> EKEEAIFRSAEMALVQFYIPQEISRDSAYTLGQLGLVQFRDLNSKVRAFQRTFVNEIRRLDNVERQYRYFYSLLKKHDIKLYEGDTDKYLDGSGELYVPPSGSVIDDYVRNASYLEERLIQMEDATDQIEVQKNDLEQYRFILQSGDEFFLKGDNTDSTSYMDEDMIDANGENIAAAIGASVNYVTGVIARDKVATLEQILWRVLRGNLFFKTVEIEQPVYDVKTREYKHKNAFIVFSHGDLIIKRIRKIAESLDANLYDVDSSNEGRSQQLAKVNKNLSDLYTVLKTTSTTLESELYAIAKELDSWFQDVTREKAIFEILNKSNYDTNRKILIAEGWIPRDELATLQARL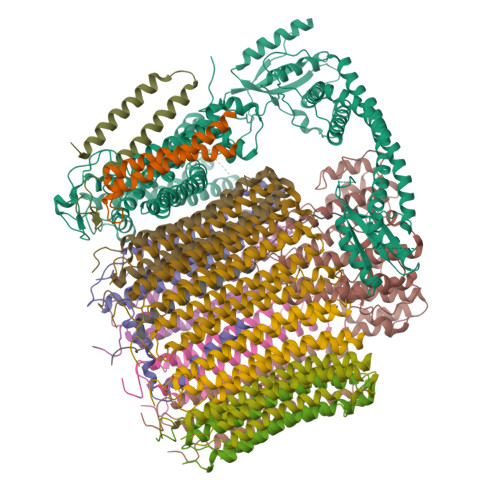GEMIARLGIDVPSIIQVLDTNHTPPTFHRTNKFTAGFQSICDCYGIAQYREINAGLPTIVTFPFMFAIMFGDMGHGFLMTLAALSLVLNEKKINKMKRGEIFDMAFTGRYIILLMGVFSMYTGFLYNDIFSKTMTIFKSGWKWPDHWKKGESITATSVGTYPIGLDWAWHGTENALLFSNSYKMKLSILMGFIHMTYSYFFSLANHLYFNSMIDIIGNFIPGLLFMQGIFGYLSVCIVYKWAVDWVKDGKPAPGLLNMLINMFLSPGTIDDELYPHQAKVQVFLLLMALVCIPWLLLVKPLHFKFTHKKKSHEPLPSTEADASSEDLEAQQLISAMDADDAEEEEVGSGSHGEDFGDIMIHQVIHTIEFCLNCVSHTASYLRLWALSLAHAQLSSVLWTMTIQIAFGFRGFVGVFMTVALFAMWFALTCAVLVLMEGTSAMLHSLRLHWVESMSKFFVGEGLPYEPFAFEYKDM;> MEGVYFNIDNGFIEGVVRGYRNGLLSNNQYINLTQCDTLEDLKLQLSSTDYGNFLSSVSSESLTTSLIQEYASSKLYHEFNYIRDQSSGSTRKFMDYITYGYMIDNVALMITGTIHDRDKGEILQRCHPLGWFDTLPTLSVATDLESLYETVLVDTPLAPYFKNCFDTAEELDDMNIEIIRNKLYKAYLEDFYNFVTEEIPEPAKECMQTLLGFEADRRSINIALNSLQSSDIDPDLKSDLLPNIGKLYPLATFHLAQAQDFEGVRAALANVYEYRGFLETGNLEDHFYQLEMELCRDAFTQQFAISTVWAWMKSKEQEVRNITWIAECIAQNQRERINNYISVY;> SFSHFLYYLVLIVVIVYGLYKLFTGHGSDINFGKFLLRTSPYMWANLGIALCVGLSVVGAAWGIFITGSSMIGAGVRAPRITTKNLISIIFCEVVAIYGLIIAIVFSSKLTVATAENMYSKSNLYTGYSLFWAGITVGASNLICGIAVGITGATAAISDAADSALFVKILVIEIFGSILGLLGLIVGLLMAGKASEFQ;> SNIYAPLYAPFFGFAGCAAAMVLSCLGAAIGTAKSGIGIAGIGTFKPELIMKSLIPVVMSGILAIYGLVVAVLIAGNLSPTEDYTLFNGFMHLSCGLCVGFACLSSGYAIGMVGDVGVRKYMHQPRLFVGIVLILIFSEVLGLYGMIVALILNTRGSE;>[8x]MTELCPVYAPFFGAIGCASAIIFTSLGAAYGTAKSGVGICATCVLRPDLLFKNIVPVIMAGIIAIYGLVVSVLVCYSLGQKQALYTGFIQLGAGLSVGLSGLAAGFAIGIVGDAGVRGSSQQPRLFVGMILILIFAEVLGLYGLIVALLLNSRATQDVV;> MSSFYTVVGVFIVVSAMSVLFWIMAPKNNQAVWRSTVILTLAMMFLMWAITFLCQLHPLVAPRRSDLRPEF;> DDILSSIWTEGLLMCLIVSALLLFILIVALSWISNLDITYGALEKSTNPIKK;> TGKAWCCTVLSAFGVVILSVIAHLFNTNHESFVGSINDPEDGPAVAHTVYLAALVYLVFFVFCGFQVYL> MAASRRLMKELEEIRKCGMKNFRNIQVDEANLLTWQGLIVPDNPPYDKGAFRIEINFPAEYPFKPPKITFKTKIYHPNIDEKGQVCLPVISAENWKPATKTDQVIQSLIALVNDPQPEHPLRADLAEEYSKDRKKFCKNAEEFT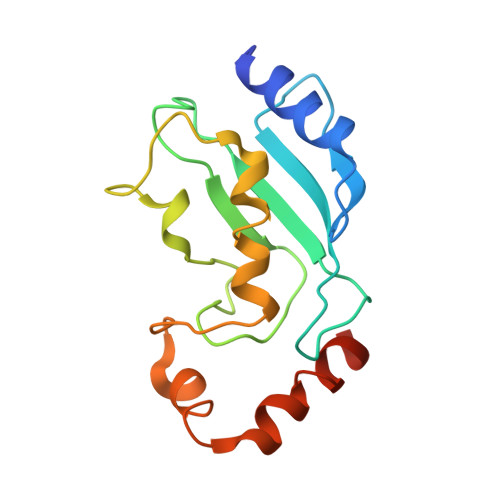KKYGEKRPVD> MALVDGFLELERSSGKLEWSAILQKMASDLGFSKILFGLLPKDSQDYENAFIVGNYPAAWREHYDRAGYARVDPVVSHCTQSVLPIFWEPSIFQTRKQHEFFEEASAAGLVYGLTMPLHGARGELGWLSLSVEAENRAEANRFMESVLPTLWMLKDYALQSGAGLAFEHPVSKPVVLTSREK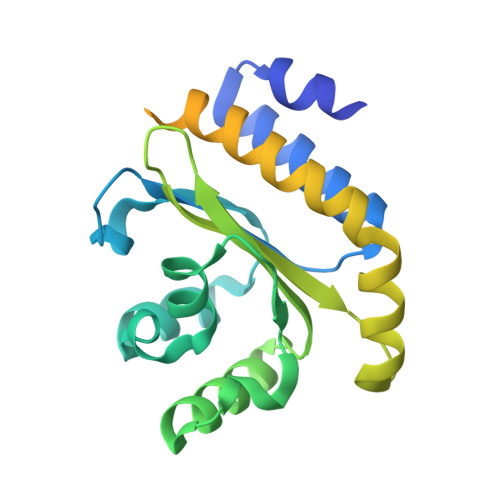EVLQWCAIGKTSWEISVICNCSEANVNFHMGNIRRKFGVTSRRVAAIMAVNLGLITL>MNDFHRDTWAEVDLDAIYDNVENLRRLLPDDTHIMASVCGNAYGHGDVQVARTALEAGASRLAVAFLDEALALREKGIEAPILVTGASRPADAALAAQQRIALTVFRSDWLEEASALYSGPFPIHFHLYMDTGMGSLGVKDEEETKRIVALIERHPHFVLEGLWTWFATADEVNTDYFSYQYTRFLHMLEW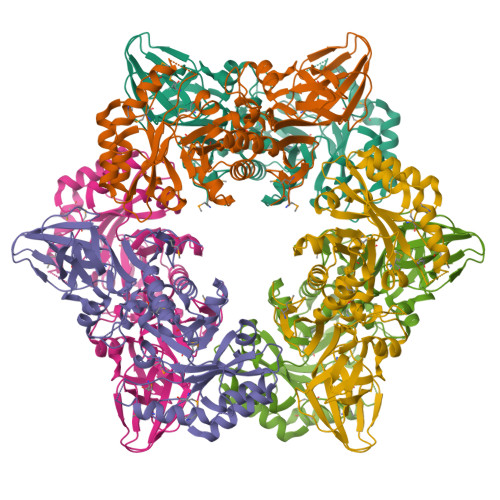LPSRPPLVHCANSAASLRFPDRTFNMVQFGIAMYGLAPSPGIKPLLPYPLKEAFSLHSRLVHVKKLQPGEKVSFGATYTAQTEEWIGTIPIGYKDGWLRRLQHFHVLVDGQKAPIVGRILGDMCMIRLPGPLPVGTKVTLIGRQGDKVISIDDVARHLETINYEVPCTISYRVPRIFFRHKRIMEVRNAIGRGESSAGS[3x]2-{5-[AMINO(IMINIO)METHYL]-1H-INDOL-2-YL}-6-BROMO-4-METHYLBENZENOLATE | C16 H14 Br N3 O | 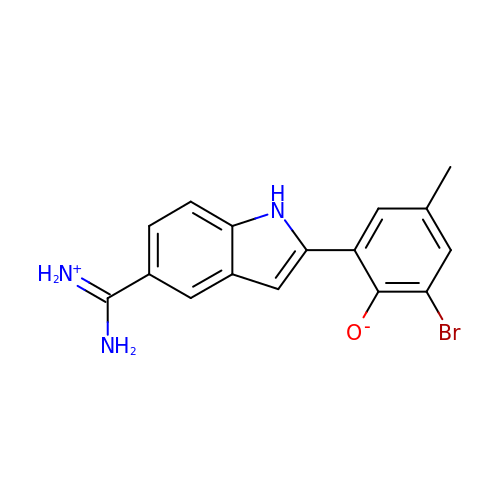BVTBOJXEAPSOEB-UHFFFAOYSA-N>[3x]TINVTGDGNVFKPSAETSSTAVPSLSLSPGMLNPGGVPWIAIGDETSVTSPGALRRMTSKDIDEPLVVVTEHAIANFTKAEMALEFNREFLDKLRVLSVSPKYSDLLTYVDCYV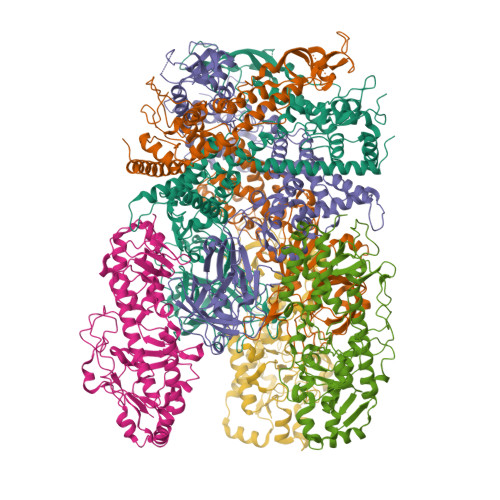GVSARQALNNFQKQVPVITPTRQTMYVDSIQAALKALEKWEIDLRVAQTLLPTNVPIGEVSCPMQSVVKLLDDQLPDDSLIRRYPKEAAVALAKRNGGIQWMDVSEGTVMNEAVNAVAASALAPSASAPPLEEKSKLTEQAMDLVTAAEPEIIASLVPVPAPVFAIPPKPADYNVRTLKIDEATWLRMIPKTMGTLFQIQVTDNTGTNWHFNLRGGTRVVNLDQIAPMRFVLDLGGKSYKETSWDPNGKKVGFIVFQSKIPFELWTAASQIGQATVVNYVQLYAEDSSFTAQSIIATTSLAYNYEPEQLNKTDPEMNYYLLATFIDSAAITPTNMTQPDVWDALLTMSPLSAGEVTVKGAVVSEVVPAELIGSYTPESLNASLPNDAARCMIDRASKIAEAIKIDDDAGPDEYSPNSVPIQGQLAISQLETGYGVRIFNPKGILSKIASRAMQAFIGDPSTIITQAAPVLSDKNNWIALAQGVKTSLRTKSLSAGVKTAVSKLSSSESIQNWTQGFLDKVSTHFPAP;>MEVCLPNGHQIVDLINNAFEGRVSIYSAQEGWDKTISAQPDMMVCGGAVVCMHCLGVVGSLQRKLKHLPHHRCNQQIRHQDYVDVQFADRVTAHWKRGMLSFVCQMHAMMNDVSPEDLDRVRTEGGSLVELNWLQVDPNSMFRSIHSSWTDPLQVVDDLDTKLDQYWTALNLMIDSSDLVPNFMMRDPSHAFNGVRLEGDARQTQFSRTFDSRSSLEWGVMVYDYSELEHDPSKGRAYRKELVTPARDFGHFGLSHYSRATTPILGKMPAVFSGMLTGNCKMYPFIKGTAKLKTVRKLVDSVNHAWGVEKIRYALGPGGMTGWYNRTMQQAPIVLTPAALTMFSDTTKFGDLDYPVMIGDPMILG[3x]>MGHHHHHHMEEAAHVKNSQCHNYAGGHVYPGEAFRVPVSDHSLHLSKAKISKPAPQWEGTAVINGEFKELKLSDYRGKYLVFFFYPLDFTFVCPTEIIAFSDRVHEFRAINTEVVACSVDSQFTHLAWIITPRKQGGLGPMKIPLLSDLTHQISKDYGVYLEDQGHTLRGLFIIDEKGVLRQITMNDLPVGRSVDETLRLVQAFQYTDKHGEVCPAGWKPGSDTIIPD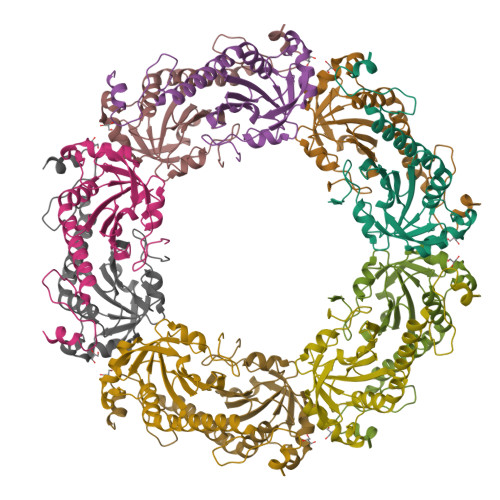PSGKLKYFDKMK[5x]> SVP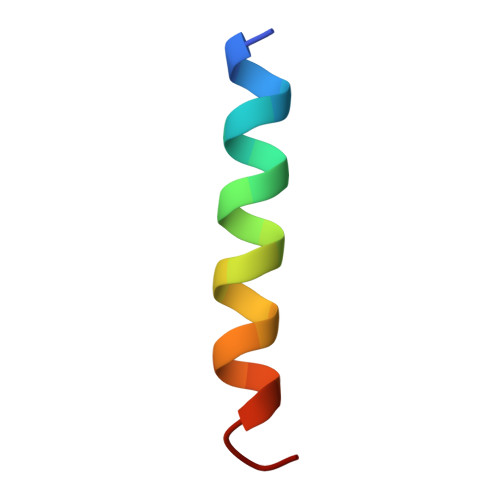QARKASLARFLEKRKERLM pentane-2,2,4,4-tetrol 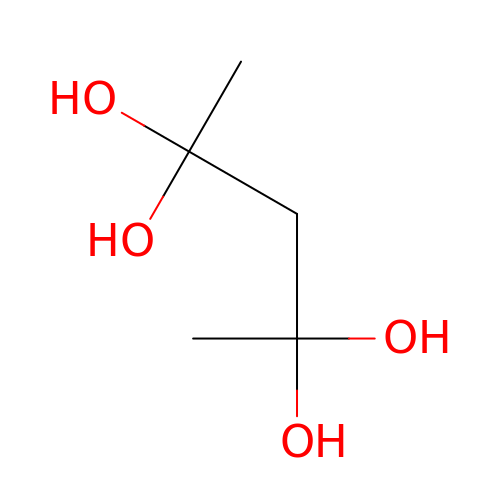| C5 H12 O4 | VNRDADQWVXLHCQ-UHFFFAOYSA-N> VLGKPQTDPTLEWFLSHCHIHKYPSKSTL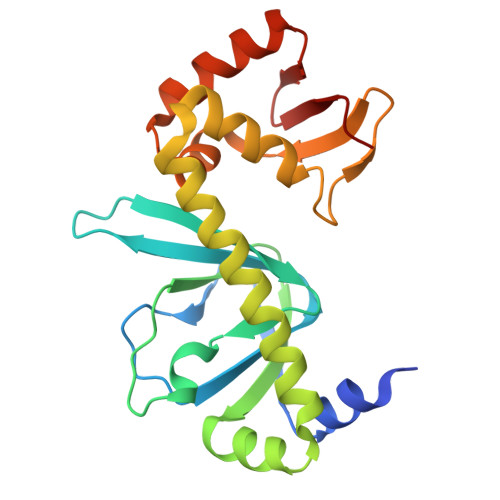IHQGEKAETLYYIVKGSVAVLIKDEEGKEMILSYLNQGDFIGELGLFEEGQERSAWVRAKTACEVAEISYKKFRQLIQVNPDILMRLSAQMARRLQVTSEKVGNLAFLDVTGRIAQTLLNLAKQPDAMTHPDGMQIKITRQEIGQIVGCSRETVGRILKMLEDQNLISAHGKTIVVYGTR>[4x]MSPFHLNDAVAIVTGAAAGIGRAIAGTFAKAGASVVVTDLKSEGAEAVAAAIRQAGGKAIGLECNVTDEQHREAVIKAALDQFGKITVLVNNAGGGGPKPFDMPMSDFEWAF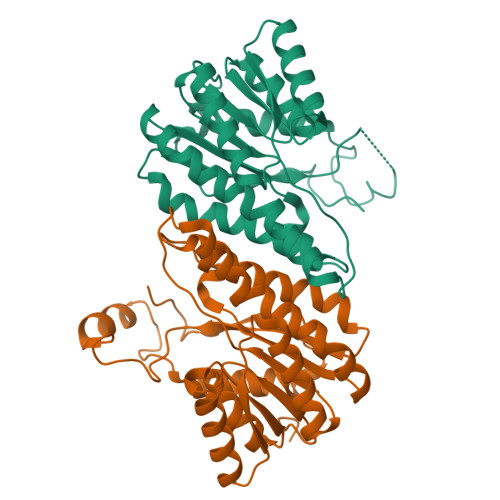KLNLFSLFRLSQLAAPHMQKAGGGAILNISSMAGENTNVRMASYGSSKAAVNHLTRNIAFDVGPMGIRVNAIAPGAIKTDALATVLTPEIERAMLKHTPLGRLGEAQDIANAALFLCSPAAAWISGQVLTVSGGGVQELD Cytoplasmic polyadenylation drives the translational activation of specific mRNAs in early metazoan development and is performed by distinct complexes that share the same catalytic poly(A)-polymerase subunit, GLD-2. GLD-2 (germline development defective 2) is a highly conserved cytoplasmic poly(A)-polymerase in metazoans. The activity and specificity of GLD-2 depend on its binding partners. In Caenorhabditis elegans, GLD-2 promotes spermatogenesis when bound to GLD-3 and oogenesis when bound to RNP-8.

We determined the structure of GLD-2PAP-D–RNP-8GB at a resolution of 2.5 Å and Rfree of 24.2%. The four independent copies of the complex in the asymmetric unit are very similar (with the exception that only two have the active site occupied by a magnesium ion and a peptide originating from a crystal-packing interaction, Supplemental Fig. 1D). The final model includes residues 544–922 of GLD-2 (with the exception of missing or disordered residues between 815–860 and 879–882) and residues 177–222 of RNP-8. RNP-8GB wraps around GLD-2PAP-D, burying more than 1800 Å2 (35%) of its accessible surface area as calculated with PISA, with extensive interactions distributed over three distinct patches. In the N-terminal half of RNP-8GB, residues 183–198 adopt an extended conformation as they stretch around the helical side of the catalytic domain (patch 1). RNP-8GB then continues with a five-turn helix that wedges in between the catalytic and central domain (patch 2). RNP-8GB ends with a short extended segment interacting with the helical domain (patch 3). First, the catalytic domain is rotated toward the central domain and has a closer conformation of the active-site cleft. In other nucleotidyl-transferases, this part of the molecule contains elements that determine the nucleotide specificity (the so-called nucleotide recognition motif or NRM [Schmidt and Norbury 2010]). Both differences are likely related to a crystallization effect: The active-site cleft binds the N-terminal residues of the RNP-8GB polypeptide of a neighboring molecule in the lattice. With hindsight, residues 177–182 of RNP-8GB mimic binding of RNA and ATP and appear essential for crystallization.

>GAMDVLSEKIWDYHNKVSQTDEMLQRKLHLRDMLYTAISPVFPLSGLYVVGSSLNGFGNNSSDMDLCLMITNKDLDQKNDAVVVLNLILSTLQYEKFVESQKLILAKVPILRINFAAPFDDITVALNANNSVAIRNTHLLCYYSSYDWRVRPLVSVVKEWAKRKGINDANKSSFTSYSLVLMVIHFLQCGPTKVLPNLQQSYPNRFSNKVDVRTLNVTMALEEVADDIDQSLSEKTTLGELLIGFLDYYANEFNYDRDAISIRQGRRVERASISNPHFWRSQWRCVCIEEPFTNSNTAHSIYDEMVFEAIKKAFREAHGELQHNHDLDKLMECEPIKA[4x];>[4x]TLFDNHPVQQYSGFNPIDFRFDDYVEGAKRFDNLANLIRSSTPTDPFANYQKPCESTSTSRSRTNSAKDQKHGP>[4x]MATVGGISDVNE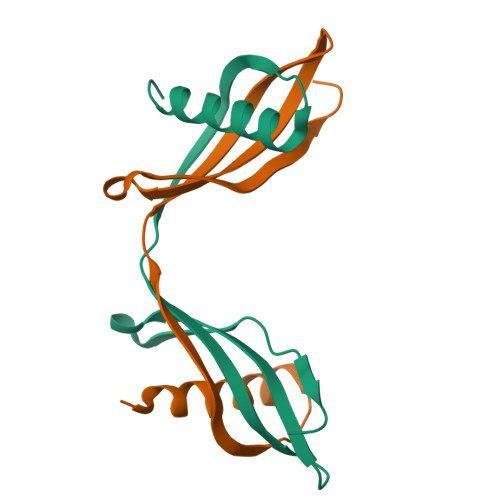GKQNSLEIDSLARFAVDEHNKKQNTLLEFGKVLNAKQQVVSGTVYYITLEVTDGGKKKVYEAKIWEKPWLNFKELQEFKLIDDAPSGSSA>MVIYGTGIDLTELSRIEAILAKGLRLPEKILTPAELAVFSRYPVKRQIEFMAGRFSAKEAYSKAYGTGIGAAVGFQDIEILDNAQGKPEVTRHPFDGPAWISISHTDTLVMTQVILERGNL[3x];>MTMDDTKATVLSILADLTGEDVSSNMDVNLFDEGILDSMGSVQLLLELQNQLGIEVPVSEFQ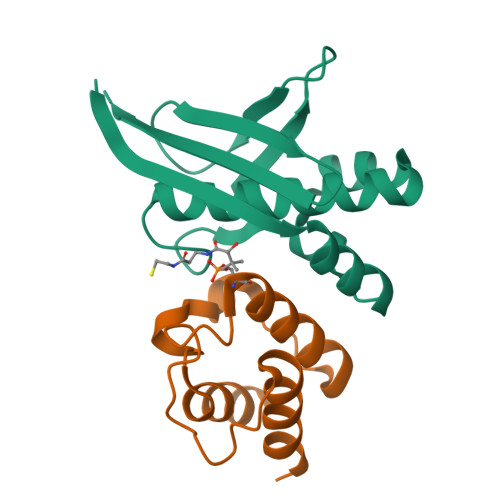RSEWDTPAKIVAKVENLQLEHHHHHH[3x]> MDFSRNLYDIGEQLDSEDLASLKFLSLDYIPQRKQEPIKDALMLFQRLQEKRM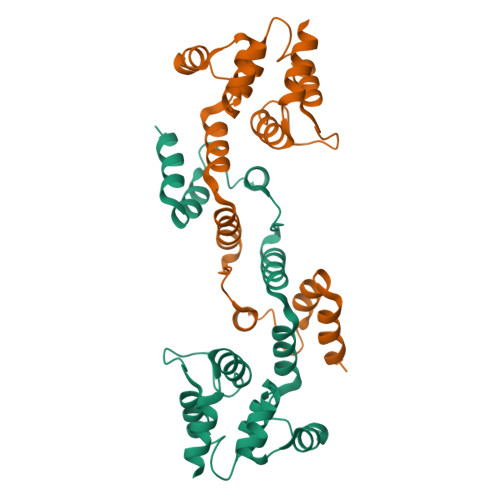LEESNLSFLKELLFRINRLDLLITYLNTRKEEMERELQTPGRAQISAYRVMLYQISEEVSRSELRSFKFLLQEEISKCKLDDDMNLLDIFIEMEKRVILGEGKLDILKRVCAQINKSLLKIINDYEEHHHHH The mutually antagonistic relationship of atypical protein kinase C (aPKC) and partitioning-defective protein 6 (Par6) with the substrate lethal giant larvae (Lgl) is essential for regulating polarity across many cell types. Although aPKC–Par6 phosphorylates Lgl at three serine sites to exclude it from the apical domain, aPKC–Par6 and Lgl paradoxically form a stable kinase–substrate complex, with conflicting roles proposed for Par6. Lgl has a double β-propeller structure and contains multiple phosphorylation sites for aPKC–Par6, with at least three serine phospho-acceptor sites (S655, S659 and S663 in human Llgl1, within a segment defined hereafter as the P-site) that map within a key membrane-binding loop13. The structure reveals the intricate interplay between aPKC–Par6 and its substrate Lgl, which, together with in vitro and in vivo data, supports a capture-and-release mechanism involving a stable phospho-intermediate.

To support these findings, we investigated how the P-site binds to aPKC in its unphosphorylated state. A peptide spanning the Llgl1 P-site is able to bind the aPKCιKD with an apparent affinity (Kd) of 48 nM. We screened for crystals of the Llgl1 and Llgl2 P-site peptides and determined a medium-resolution structure for the Llgl2 P-site peptide spanning residues 634–662 bound to aPKCιKD in the absence of nucleotide. The Llgl2 P-site is identical to the Llgl1 sequence in this region but is ten residues shorter in numbering. The cocrystal structure of aPKCιKD–Llgl2P-site revealed ordered contacts between residues 650 and 656 of the Lgl P-site, including the C-terminal S653 (equivalent to Llgl1 S663). In this poise, Llgl2S653 is bound ready for phospho-transfer, with Llgl2F654 in the hydrophobic +1 pocket. The R655 side chain forms a hydrogen bond with the G398 carbonyl and a phosphate oxygen from phospho-T412, while the R651 side chain at the −2 position, relative to the phospho-acceptor, lies in a pocket formed between Y419 and E445 of aPKCι. The structure confirms that the Lgl P-site binds aPKC, thereby presenting Llgl2S653 (equivalent to Llgl1S663) for initial phosphorylation, consistent with the cryo-EM structure. Absent from the X-ray structure is the L640-S641-R642 motif, suggesting that this motif may not be crucial for the initial C-terminal Llgl1 and Llgl2 phosphorylation. Thus, we can predict the phosphorylation trajectory from snapshots of unphosphorylated peptide (X-ray structure) to a stalled initial site phosphorylation (cryo-EM structure), as well as the S655 and S659 phosphorylation binding poses, on the basis of related substrate peptide structures.

>ESGKASSSLGLQDFDLLRVIGRGSYAKVLLVRLKKTDRIYAMKVVKKELVNDDEDIDWVQTEKHVFEQASNHPFLVGLHSCFQTESRLFFVIEYVNGGDLMFHMQRQRKLPEEHARFYSAEISLALNYLHERGIIYRDLKLDNVLLDSEGHIKLTDYGMCKEGLRPGDTTSTFCGTPNYIAPEILRGEDYGFSVDWWALGVLMFEMMAGRSPFDIVGSSDNPDQNTEDYLFQVILEKQIRIPRSLSVKAASVLKSFLNKDPKERLGCHPQTGFADIQGHPFFRNVDWDMMEQKQVVPPFKPNISGEFGLDNFDSQFTNEPVQLTPDDDDIVRKIDQSEFEGFEYINPLLMSAEECV[2x];>[2x]SRVKSLKKSLRQSFRRMRKS>[4x]MSTQKNARATAGEVEGSDALRMDADRAEQCVDALNADLANVYVLYHQ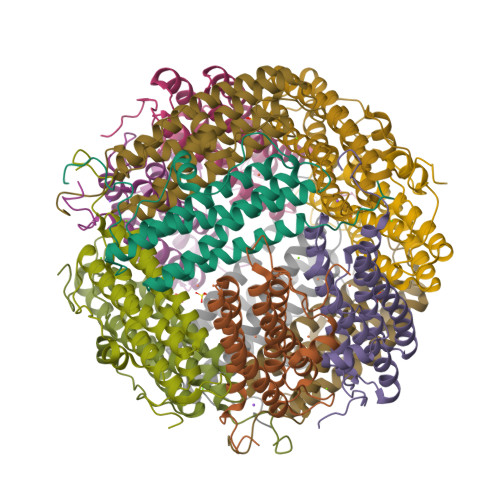LKKHHWNVEGAEFRDLHLFLGEAAETAEEVADELAERVQALGGVPHASPETLQAEASVDVEDEDVYDIRTSLANDMAIYGDIIEATREHTELAENLGDHATAHMLREGLIELEDDAHHIEHYLEDDTLVTQGALE(2S)-2-[({4-[(2-amino-7H-pyrrolo[2,3-d]pyrimidin-4-yl)oxy]phenyl}carbamoyl)amino]-4-phenylbutanoic acid | C23 H22 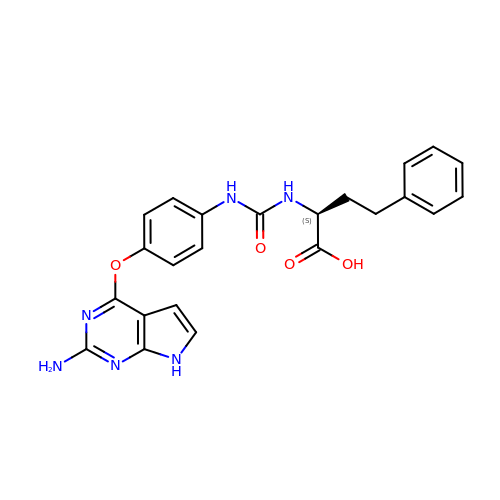N6 O4 | PCOWASOBSDEANU-SFHVURJKSA-N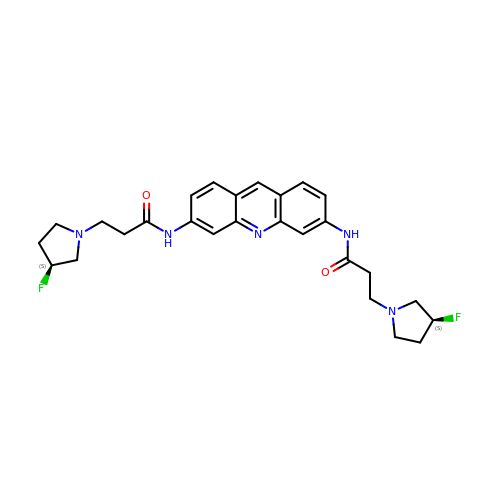3,6-bis(3-(3'-(S)-fluoropyrrolindino)propionamido)acridine | C27 H31 F2 N5 O2 | LWWRDCOEZPEHNJ-SFTDATJTSA-N>SADRAASDLLIGMFGSVSLVNLLTIIGCLWVLRVTRPPVSVMIFTWNLVLSQFFSILATMLSKGIMLRGALNLSLCRLVLFVDDVGLYSTALFFLFLILDRLSAISYGRDLWHHETRENAGVALYAVAFAWVLSIVAAVPTAATGSLDYRWLGCQIPIQYAAVDLTIKMWFLLGAPMIAVLANVVELAYSDRRDHVWSYVGRVCTFYVTCLMLFVPYYC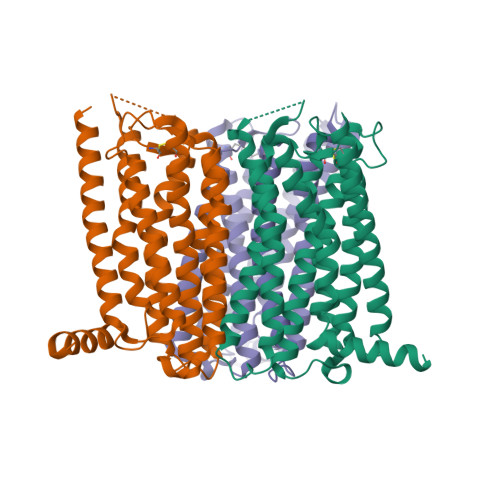FRVLRGVLQPASAAGTGFGIMDYVELATRTLLTMRLGILPLFIIAFFSREPTKDLDDSFDYLVERC[3x]>MKYLVLVLCLTSCACRDIGLWTFRYVYNESDNVVFSPYGLTSALSVLRIAAGGNTKREIDVPESVVEDSDAFLALRELFVDASVPLRPEFTAEFSSRFNTSVQRVTFNSENVKDVINSYVKDKTGGDVPRVLDASLDRDTKMLLLSSVRMKTSWRHVFDPSFTTDQPFYSGNVTYKVRMMNKIDTLKTETFTLRNVGYSVTELPYKRRQTAMLLVVPDDLGEIVRALDLSLVRFWIRNMRKDVCQVVMPKFSVESVLDLRDALQRLGVRDAFDPSRADFGQASPSNDLYVTKVLQTSKIEADERGTTASSDTAIT[3x];>[3x]LIPRNALTAIVANKPFMFLIYHKPTTTVLFMGTITKGE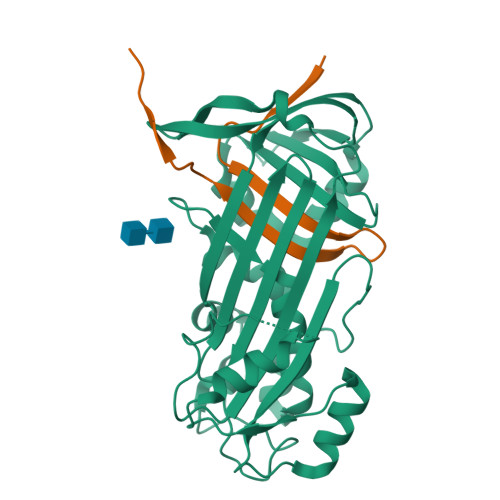KVIYDTEGRDDVVSSV>TRDQNGTWEMESNENFEGYMKALDIDFATRKCAVRLTQTKVIDQDGDNFKDKTTSTFRNYDVDFTVGVEFDEYTKSLDNRH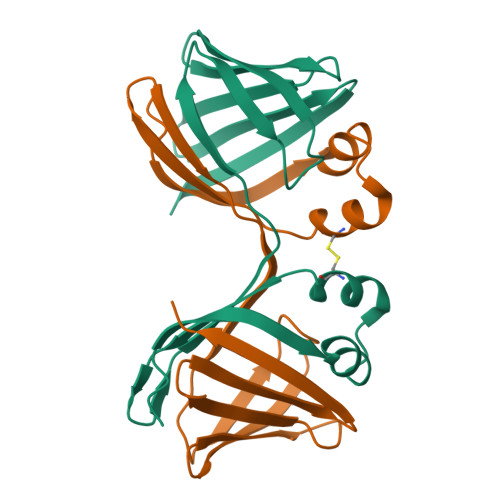VKALVTWEGDVLVCVQKGEKENRGWKKWIEGDKLYLELTCGDQVCRQVFKKK[2x]>[3x]GSHMPGFYEIVIKVPSDLDEHLPGISDSFVNWVAEKEWELPPDSDMDLNLIEQAPLTVAEK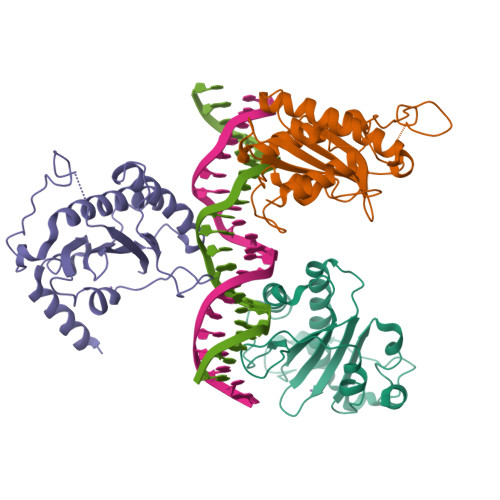LQRDFLTEWRRVSKAPEALFFVQFEKGESYFHMHVLVETTGVKSMVLGRFLSQIREKLIQRIYRGIEPTLPNWFAVTKTRNGAGGGNKVVDESYIPNFLLPKTQPELQWAWTNMEQYLSACLNLTERKRLVAQHLTHVSQTQEQNKENQN>MAKKTSGRGKLPPGPTPLPVIGNILQIGIKDISKSLTNLSKVYGPVFTLYFGLKPIVVLHGYEAVKEALIDLGEEFSGRGIFPLAERANRGFGIVFSNGKKWKEIRRFSLMTLRNFGMGKRSIEDCVQEEARCLVEELRKTKASPCDPTFILGCAPCNVICSIIFHKRFDYKDQQFLNLMEKLNENIKILSSPWIQICNNFSPIIDYFPGTHNKLLKNVAFMKSYILEKVKEHQESMDMNNPQDFIDCFLMKMEKEKHNQPSEFTIESLENTAVDLFGAGTETTSTTLRYALLLLLKHPEVTAKV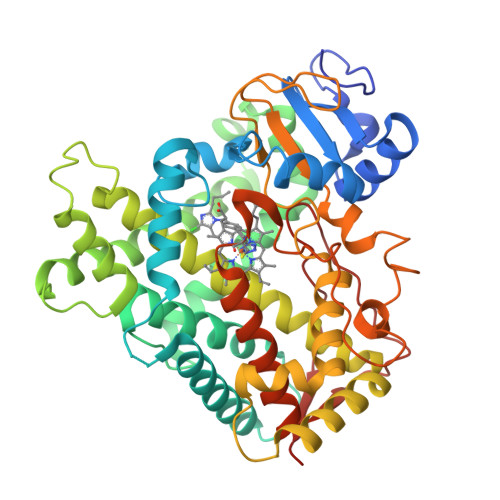QEEIERVIGRNRSPCMQDRSHMPYTDAVVHEVQRYIDLLPTSLPHAVTCDIKFRNYLIPKGTTILISLTSVLHDNKEFPNPEMFDPHHFLDEGGNFKKSKYFMPFSAGKRICVGEALAGMELFLFLTSILQNFNLKSLVDPKNLDTTPVVNGFASVPPFYQLCFIPIHHHH[8x]>[2x]GVE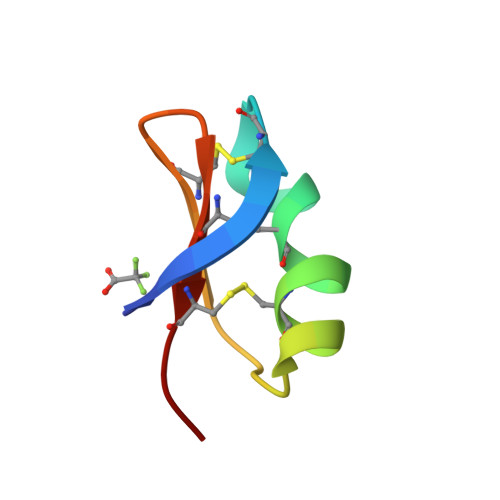INVKCSGSPQCLKPCKDAGMRFGKCMNRKCHCTPK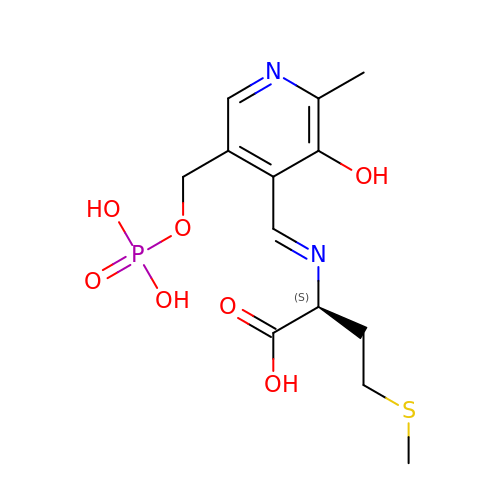N-[(3-HYDROXY-2-METHYL-5-{[(TRIHYDROXYPHOSPHORANYL)OXY]METHYL}PYRIDIN-4-YL)METHYLENE]METHIONINE | C13 H19 N2 O7 P S | HPCOPQVFKQIVQF-DMSFABOWSA-N> MHISKKKGVRKMNLDMIIQFIVLGGIILSSVLMIVTRDLLVAVLASAAMSLLLSLEFYMLHAPDVAIAEAAVGAGVVTALVMYAISKTERWE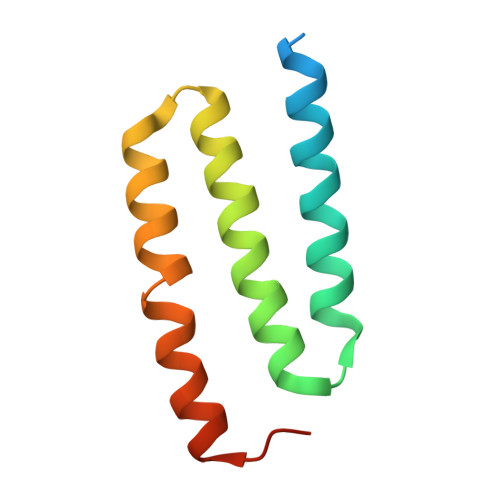REAP5-chloro-2-methoxy-4[(1Z)-3-(4-methoxyphenyl)-3-oxoprop-1-en-1-yl]aminobenzoic 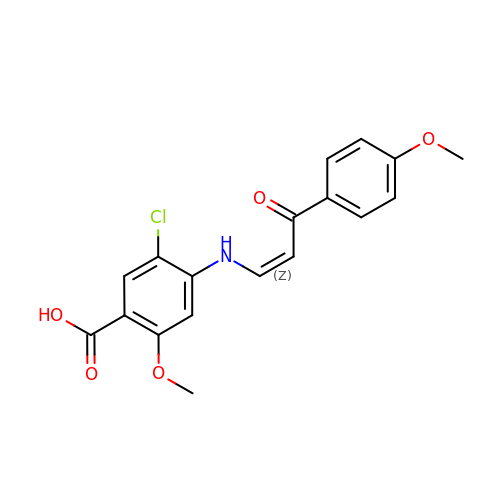acid | C18 H16 Cl N O5 | KFXXLYWMHLDCLE-FPLPWBNLSA-N> LQ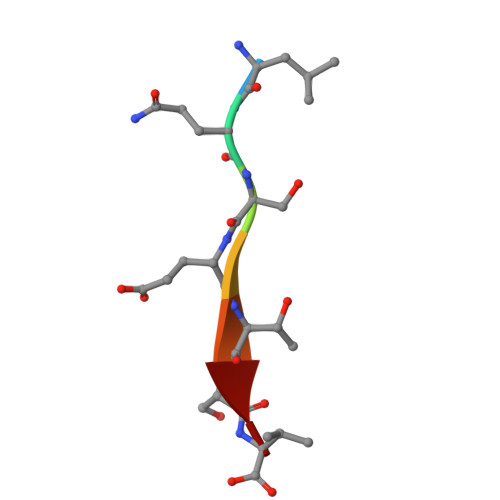SETSV> MHHHHHHHHE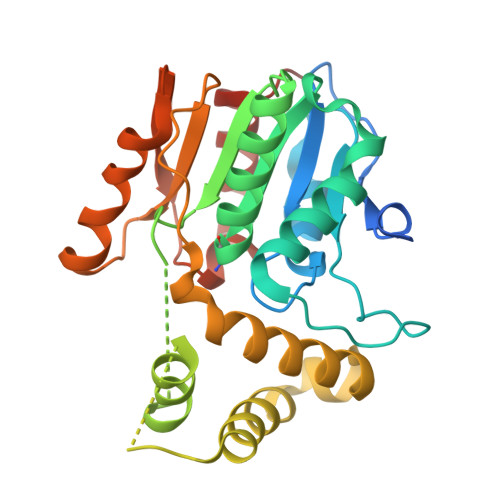NLYFQGGSSTAGDPTAKLVRLNPRGGDGPGIVFAPPAGGTVLGYIELARHLKGFGEIHGVEAPGLGAGETPVYPSFEEMVQFCSDSAAGVAGDGVYIGGHALGGHIAFYLATMLLDRGIRPKGLIILDTPPRLGDIPVADADLTEEETKVFILAMGIGGMLDQDRDALKDLPYEEAKQLLLDRAKNDPRVSAFLSEDYLDRFLRLQMHQLMYSRDVVLPQRKLDIPIHVFRTKNHAPEVARLFSAWENYAAGEVTFVDIPGDHATMLRAPHVSEVAQLLDRHCGLPSDDGPRG> SDMPVERILEAELAVEPKTETYVEANMGLNPSSPNDPVTNICQAADKQLFTLVEWAKRIPHFSELPLDDQVILLRAGWNELLIASFSHRSIAVKDGILLATGLHVHRNSAHSAGVGAIFDRVLTEL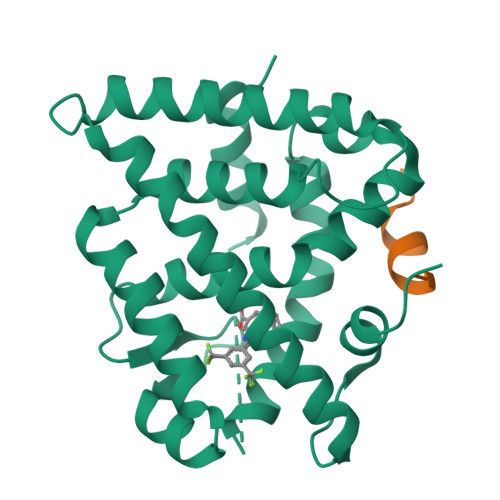VSKMRDMQMDKTELGCLRAIVLFNPDSKGLSNPAEVEALREKVYASLEAYCKHKYPEQPGRFAKLLLRLPALRSIGLKCLEHLFFFKLIGDTPIDTFLMEMLEAPHQMT;> HKILHRLLQD> SPSAEACGYSDRVAQLTIGNSTITTQEAANIVIAYGEWPEYCPDTDATAVDKPTRPDVSVNRFFTLDTKSWAKDSKGWYWKFPDVLTE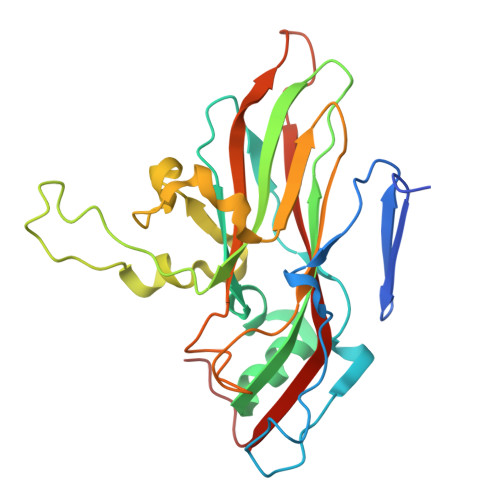VGVFGQNAQFHYLYRSGFCVHVQCNASKFHQGALLVAVLPEYVLGTIAGGTGNENSHPPYATTQPGQVGAVLTHPYVLDAGIPLSQLTVCPHQWINLRTNNCATIIVPYMNTVPFDSALNHCNFGLLVIPVVPLDFNTGATSEIPITVTIAPMCAEFAGLRQAVKQ> MGHHHHHHHHHHGENLYFQGFGDGGGAPS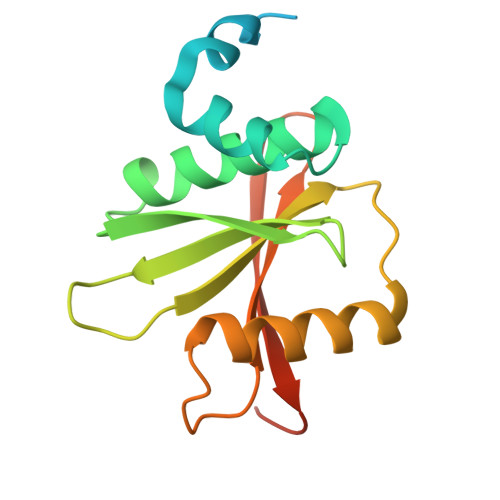WAPEDAWMGTHPKYLEMMELDIGDATQVYVAFLVYLDLMESKSWHEVNCVGLPELQLICLVGTEIEGEGLQTVVPTPITASLSHNRIREILKASRKLQGDPDLPMSFTLAIVESDSTIVYYKLTDGFMLPDPQNISLR>MEEEVREKLKRMEKKFDDSLEKAERKIREIIKEAEKKLKTLKKRNGPYEAVVTTLRAILKAVETKIRAIIKALKTELDALIKAMETILKAHDKNDELKKEVEDIIKKMRDKLTKLIRKAKELLDRLKKKAKK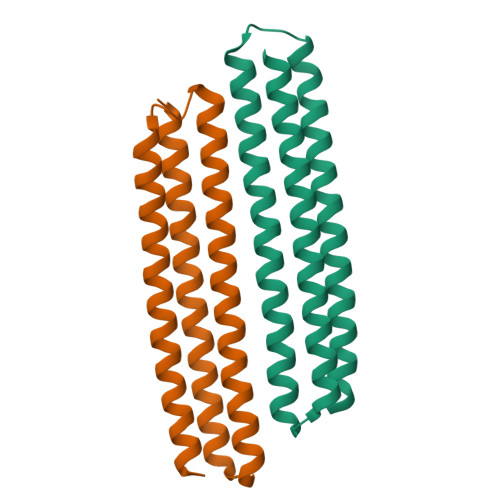VQDETSGGW[2x]>MTRLDSVERAVADIAAGKAVIVIDDEDRENEGDLIFAAEKATPEMVAFMVRYTSGYLCVPLDGAICDRLGLLPMYAVNQDKHGTAYTVTVDARNGIGTGISASDRATTMRLLADPTSVADDFTRPGHVVPLRAKDGGVLRRPGHTEAAVDLARMAGLQPAGAICEIVSQKDEGSMAHTDELRVFADEHGLALITIADLIEWRRKHEKHIERVAEARIPTRHGEFRAIGYTSIYEDVEHVALVRGEIAGPNADGDDVLVRVHSECLTGDVFGSRRCDCGPQLDAALAMVAREGRGVVLYMRGHEGRGIGLMHKLQAYQLQDAGADTVDANLKLGLPADARDYGIGAQILVDLGVRSMRLLTNNPAKRVGLDGYGLHIIERVPLPVRANAENIRYLMTKRDKLGHDLAGLDDFHESV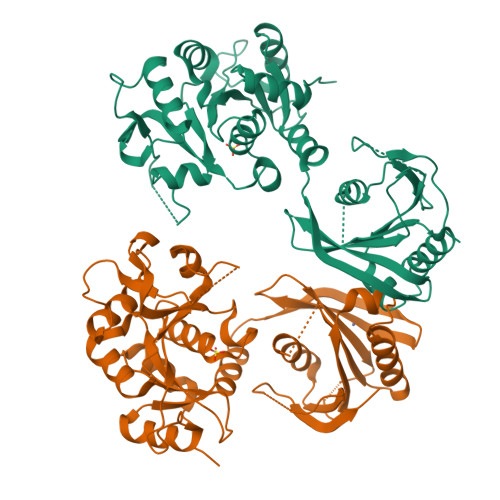HLPGEFGGAL[2x]5'-O-[(R)-hydroxy{[(R)-hydroxy{[(S)-hydroxy(phosphonooxy)phosphoryl]oxy}phosphoryl]oxy}phosphoryl]-7-methylguanosine 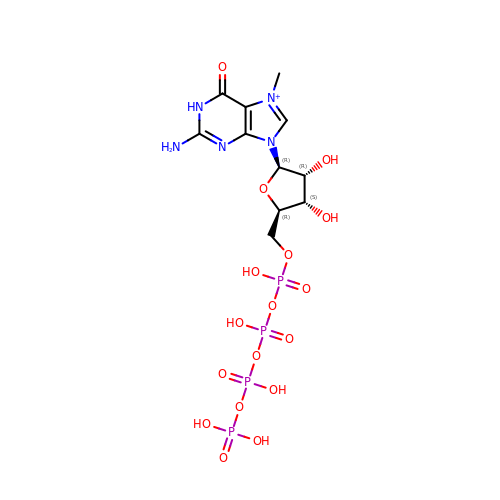| C11 H20 N5 O17 P4 | ICYVMAXYRWTAKS-KQYNXXCUSA-O> MAKATKEVKSKRVEALRQVAYQRLERLERKAQKIGAHLRKPGKAADLQSLHYLLHKVEVEYHDIARNLEKDPTWTPKPKMRREKRAIVPESGPAAPLPTTAKGEPGRPANRHIPPPVPLDSARIPEDQQSMGQGSGGRSWCSAPFVEVKLPPTQWSNVREKLLKFRIEDDADIVRRWAEAKFGSIETARDGLRASAEIGTSPDVWRSFISRAISNGKKDFEPLLSLDDDELTADATAERVVRRWHQIDWVGRMLDSILETVPSGVSKDTFRSRVESRLKTFHSSVNSFELKKRKDGTVERKRKHTNPQFPYLSPSAVSIDPDVVTMEAVELLQMQPEERFAKDPNDANGRMRLRVLQAELGKARREALGRRGEKAPPWSGRKVFRGTTTRKREACLVWDKEAQADGLYFALVMSGGPKIDDKRFVYMDGQPLQSDWQLHNGVAGKAKSCRAMPLILKHDFLRWYHRHIKNHDVNAPLEKRCVHTTTQFVFVEPDEKKGLQPRLFIRPVFKFYDPVYEVPDSHSIDKKPDCRYLIGIARGVNYPYRAAVYDCETNSIIADKFVDGRKADWERIRNELAYHQRRRDLLRNSRASSAAIQREIRAIARIRKRERGLNKVETVESIARLVDWAEENLGKCNYCFVLADLSSNLNLGRNNRVKHIAAIKEALINQMRKRGYRFKKSGKVDGVREESAWYTSAVAPSGWWAKKEEVDGAWKADKTRPLARKIGSYYCCEEIDGLHLRGVLKGLGRAKRLVLQSDDPSAPTRRRGFGSELFWDPYCTELCGHAFPQGVVLDADFIGAFNIALRPLVREELGKKAKAVDLADR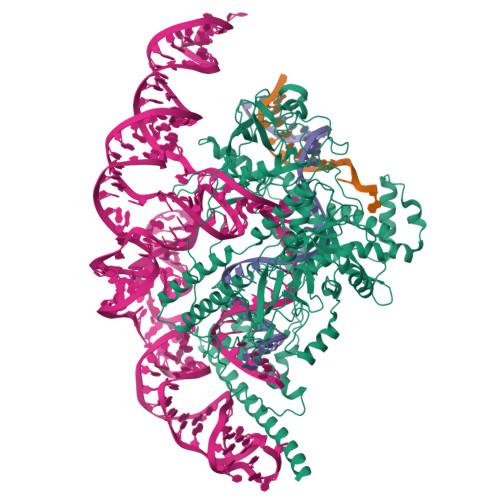HQTLNPTVALRCGVTAYEFVEVGGDPRGGLRKILLNPAEAVI~{tert}-butyl ~{N}-[(2~{S},3~{R},5~{R})-6-[[(2~{S})-1-[[(2~{S})-1-azanyl-1-oxidanylidene-3-phenyl-propan-2-yl]amino]-4-methyl-1-oxidanylidene-pentan-2-yl]amino]-3-oxidanyl-6-oxidanylidene-1-phenyl-5-(phenylmethyl)hexan-2-yl]carbamate 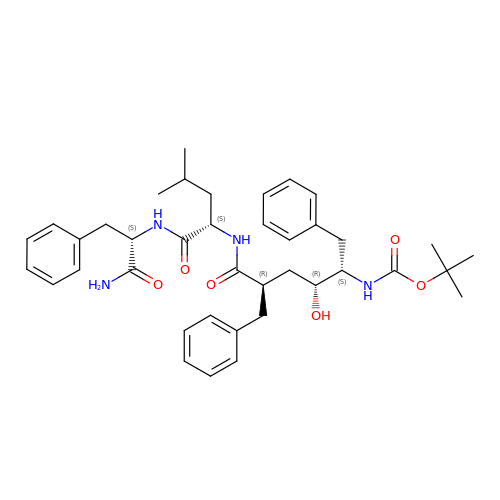| C39 H52 N4 O6 | MURCDOXDAHPNRQ-ZJKZPDEISA-N>[2x]MIKVRVPDFSDKKFSDRWRYCVGTGRLGLALQKEYIETLKYVKENIDFKYIRGHGLLCDDVGIYREDVVGDEVKPFYNFTYIDRIFDSFLEIGIRPFVEIGFMPKKLASGTQTVFYWEGNVTPPKDYEKWSDLVKAVLHHFISRYGIEEVLKWPFEIWNEPNLKEFWKDADEKEYFKLYKVTAKAIKEVNENLKVGGPAICGGADYWIEDFLNFCYEENVPVDFVSRH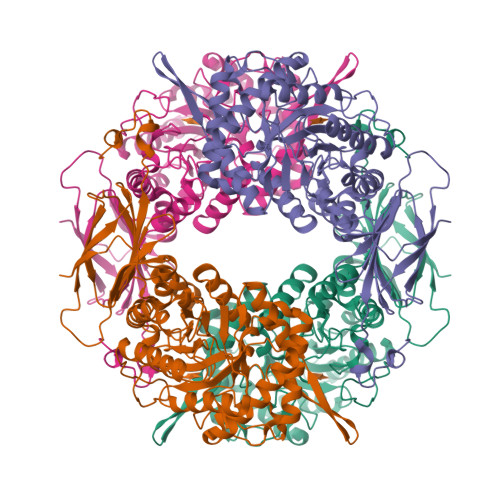AYTSKQGEYTPHLIYQEIMPSEYMLNEFKTVREIIKNSHFPNLPFHITEYNTSYSPQNPVHDTPFNAAYIARILSEGGDYVDSFSYWTFSDVFEERDVPRSQFHGGFGLVALNMIPKPTFYTFKFFNAMGEEMLYRDEHMLVTRRDDGSVALIAWNEVMDKTENPDEDYEVEIPVRFRDVFIKRQLIDEEHGNPWGTWIHMGRPRYPSKEQVNTLREVAKPEIMTSQPVANDGYLNLKFKLGKNAVVLYELTERIDESSTYIGLDDSKINGY>[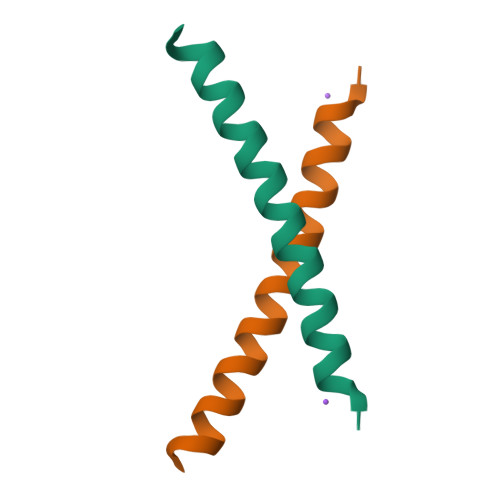2x]SVSEIQLMHNLGKHLNSMERVEWLRKKLQDVHNF>MFALGLPFLVLLVASVESHLGVLGPKNVSQKDAEFERTYVDEVNSELVNIYTFNHTVTRNRTEGVRVSVNVLNKQKGAPLLFVVRQKEAVVSFQVPLILRGMFQRKYLYQKVERTLCQPPTKNESEIQFFYVDVSTLSPVNTTYQLRVSRMDDFVLRTGEQFSFNTTAAQPQYFKYEFPEGVDSVIVKVTSNKAFPCSVISIQDVLCPVYDLDNNVAFIGMYQTMTKKAAITVQRKDFPSNSFYVVVVVKTEDQACGGSLPFYPFAEDEPVDQGHRQKTLSVLVSQAVTSEAYVSGMLFCLGIFLSFYLLTVLLACWENWRQKKKTLLVAIDRACPESGHPRVLADSFPGSSPYEGYNYGSFENVSGSTDGLVDSAGTGDLSYGYQGRSFEPVGTRPRVDSMSSVEEDDYDTLTDIDSDKNVIRTKQYLYVADLARKDKRVLRKKYQIYFWNIATIAVFYALPVVQLVITYQTVVNVTGNQDICYYNFLCAHPLGNLSAFNNILSNLGYILLGLLFLLIILQREINHNRALLRNDLCALECGIPKHFGLFYAMGTALMMEGLLSACYHVCPNYTNFQFDTSFMYMIAGLCMLKLYQKRHPDINASAYSAYACLAIVIFFSVLGVVFGKGNTAFWIVFSIIHIIATLLLSTQLYYMGRWKLDSGIFRRILHVLYTDCIRQCSGPLYVDRMVLLVMGNVINWSLAAYGLIMRPNDFASYLLAIGICNLLLYFAFYIIMKLRSGERIKLIPLLCIVCTSVVWGFALFFFFQGLSTWQKTPAESREHNRDCILLDFFDDHDIWHFLSSIAMFGSFLVLLTLDDDLDTVQRDKIYVF[2x]

The systemic RNAi-defective (SID) transmembrane family member 2 (SIDT2) is a putative nucleic acid channel or transporter that plays essential roles in nucleic acid transport and lipid metabolism. Here, we report the cryo-electron microscopy (EM) structures of human SIDT2, which forms a tightly packed dimer with extensive interactions mediated by two previously uncharacterized extracellular/luminal β-strand-rich domains and the unique transmembrane domain (TMD). The TMD of each SIDT2 protomer contains eleven transmembrane helices (TMs), and no discernible nucleic acid conduction pathway has been identified within the TMD, suggesting that it may act as a transporter. Notably, SIDT2 can hydrolyze C18 ceramide into sphingosine and fatty acid with a slow rate.

The apoSIDT2-pH 7.4, apoSIDT2-pH 5.5, and SIDT2-pH 5.5 plus miRNA structures were determined at overall resolutions of 3.16 Å, 3.21 Å, and 2.87 Å, respectively. No reliable RNA density was observed in the map of SIDT2-pH 5.5 plus miRNA, and no conformational change was found in any of these structures; therefore, we used the SIDT2-pH 5.5 plus miRNA structure with the highest resolution of 2.87 Å for structural analysis. The 2.87 Å EM map displays excellent main chain connectivity and side chain densities for almost all residues of the extracellular/luminal domain (ECD) of SIDT2. Notably, the only difference in these three structures is that an additional dense area is observed in the map of SIDT2-pH 5.5 plus miRNA in the region that, on the basis of the AF-SIDT2 structure, was expected to be the CTD. An additional area of density with extremely low resolution was observed in the map of SIDT2-pH 5.5 plus miRNA, we cannot reliably distinguish whether it belongs to the protein or the RNA. Based on the structure of AF-SIDT2, a portion of the CTD was predicted to be located in the dimer interface, suggesting that the additional area of density is more likely a portion of the CTD. It has been reported that an arginine-rich motif in the CTD is capable of binding nucleic acids. As the CTD is unresolved in the maps of SIDT2 alone samples, reflecting its intrinsic flexibility, the binding of RNA may stabilize this region.>GMENIEYVFEDVVRIYDTDAQGIAHYAAYYRFFTNTIEKFIKEKVGIPYP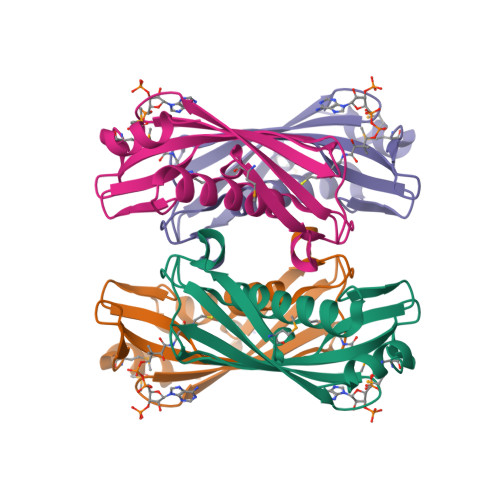IVNENLWFVIAESHAIYHRPVKLGDKLTVLLNPKILSNKTIKFEFKVLKDGELTTEGYVIQIAINPKIWKSTEMPKEIMDKLSIK[4x]>[2x]MNSEEVNDIKRTWEV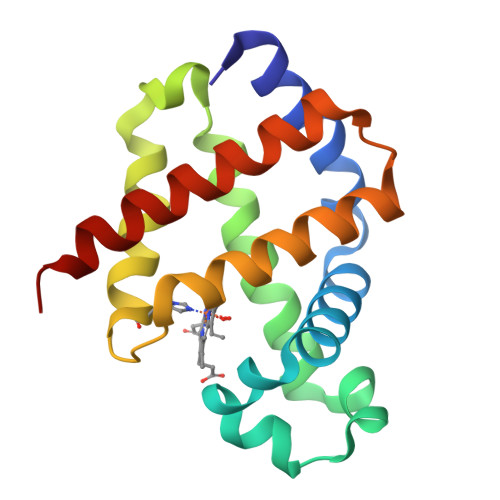VAAKMTEAGVEMLKRYFKKYPHNLNHFPWFKEIPFDDLPENARFKTHGTRILRQVDEGVKALSVDFGDKKFDDVWKKLAQTHHEKKVERRSYNELKDIIIEVVCSCVKLNEKQVHAYHKFFDRAYDIAFAEMAKMG> MKIAVAGSGYVGLSLGVLLSLQNEVTIVDILPSKVDKINNGLSPIQDEYIEYYLKSKQLSIKATLDSKAAYKEAELVIIATPTNYNS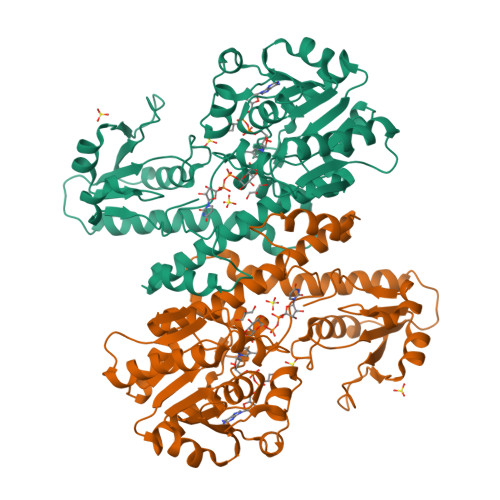RINYFDTQHVETVIKEVLSVNSHATLIIKSTIPIGFITEMRQKFQTDRIIFSPEFLRESKALYDNLYPSRIIVSCEENDSPKVKADAEKFALLLKSAAKKNNVPVLIMGASEAEAVKLFANTYLALRVAYFNELDTYAESRKLNSHMIIQGISYDDRIGMHYNNPSFGYGGYSLPKDTKQLLANYNNIPQTLIEAIVSSNNVRKSYIAKQIINVLKEQESPVKVVGVYRLIMKSNSDNFRESAIKDVIDILKSKDIKIIIYEPMLNKLESEDQSVLVNDLENFKKQANIIVTNRYDNELQDVKNKVYSRDIFGRD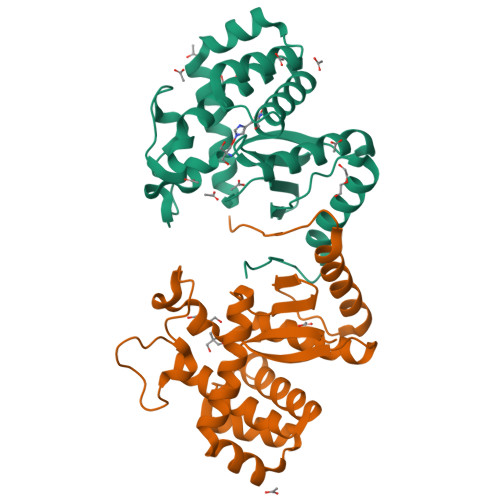>MHHHHHHTPQPTDAQPTDAQPTDLYFDFLSPYAWRGVEMAHVLRGSGEGFRLRHFSLVQGNHPQNKDQETVQWWLTDQPLGAEGGSGYMKYQRPSLNAFLAAHAAARQGEEKSWAFALALFRLHHEDKRDLDEAAFQDAATRAGLDLSQWKQDRQDEAGLRRELRADLEAAAALGVFGTPTFDLGGGDVAYFKFEELTRDPQAARDLWNLFTSTLRSEARVATIRRPVPKKG[2x]> SNTNVPIFSSPVRDLPRSFEQKHLAVVDAFFQTYHVKPDFIARSPGRVNLIGEHIDYCDFSVLPLAIDVDMLCAVKILDEKNPSITLTNADPKFAQRKFDLPLDGSYMAIDPSVSEWSNYFKCGLHVAHSYLKKIAPERFNNTPLVGAQIFCQSDIPTGGGLSSAFTCAAALATIRANMGKNFDISKKDLTRITAVAEHYVGVNNGGMDQATSVYGEEDHALYVEFRPKLKATPFKFPQLKNHEISFVIANTLVKSNKFETAPTNYNLRVIEVTVAANALATRYSVALPSHKDNSNSERGNLRDFMDAYYARYENQAQPWNGDIGTGIERLLKMLQLVEESFSRKKSGFTVHEASTALNCSREEFTRDYLTTFPVRFQVLKLYQRAKHVYSESLRVLKALKMMTSATFHTDEDFFTDFGRLMNESQASCDKLYECSCIETNQICSIA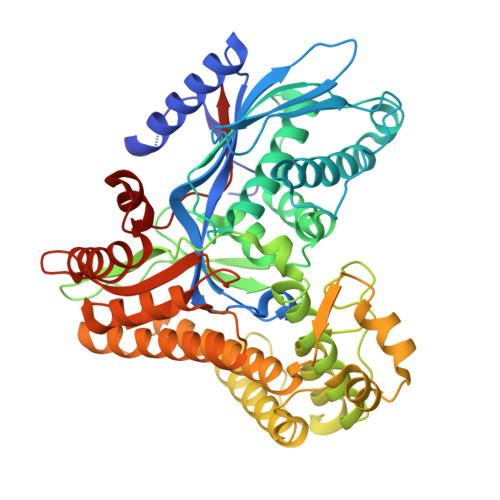LANGSFGSRLTGAGWGGCTIHLVPSGANGNVEQVRKALIEKFYNVRYPDLTDEELKDAIIVSKPALGTCLYEQ>SMTDEYQLFEELGKGAFSVVRRCMKIPTGQEYAAKIINTKKLSARDHQKLEREARICRLLKHPNIVRLHDSISEEGFHYLVFDLVTGGELFEDIVAREYYS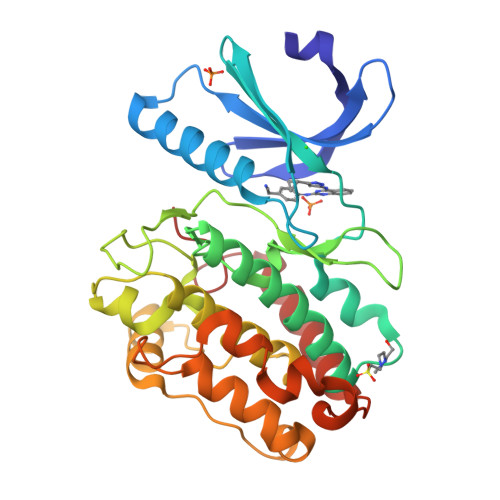EADASHCIQQILESVNHCHLNGIVHRDLKPENLLLASKSKGAAVKLADFGLAIEVQGDQQAWFGFAGTPGYLSPEVLRKDPYGKPVDMWACGVILYILLVGYPPFWDEDQHRLYQQIKAGAYDFPSPEWDTVTPEAKDLINKMLTINPAKRITASEALKHPWICQRSTVASMMHRQETVDCLKKFNARRKLKGAILTTML[2x]>[6x]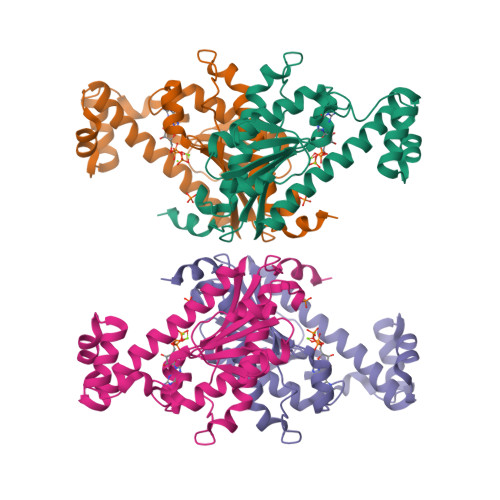MANSKFGYVRQFETHDVILPQCYIVVRIDGKKFHEFSKFYEFAKPNDENALKLMNACAKNLVLKYKNDIILAFGESDEYSFILKSSTTLFNRRKDKLATLFGSFFTSNYVALWAKFFPEKPLNIKHLPYFDSRCVAYPNLQTIKDYLSWRYVDTHINNLYNTTFWQLIIKCGLTPQESEKKLCGTFSNEKQEILFSECGINYNNEPEMFKKGSLVTRKGEILHINVIAQIDELFEGYHHHHHH>[2x]MLIAFEGIDGSGKTTQAKKLYEYLKQKGYFVSLYREPGGTKVGEVLREILLTEELDERTELLLFEASRSKLIEEK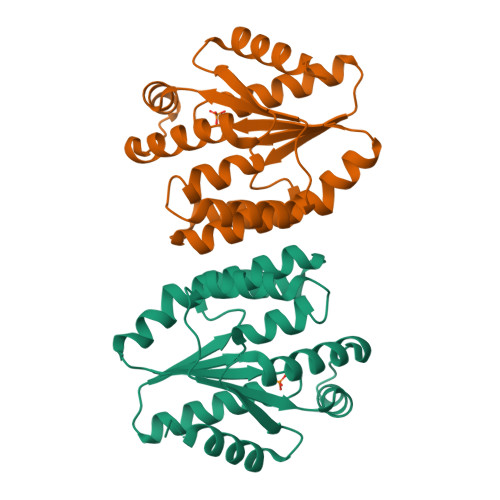IIPDLKRDKVVILDAFVLSTIAYQGYGKGLDVEFIKNLNEFATRGVKPDITLLLDIPVDIALRRLKEKNRFENKEFLEKVRKGFLELAKEEENVVVIDASGEEEEVFKEILRALSGVLRV>MDFKYTEEKELIKINNVMIHKYTILYTSNCILDISFGEDKITCFNNRLVFLERGVNISVRIQKQKLT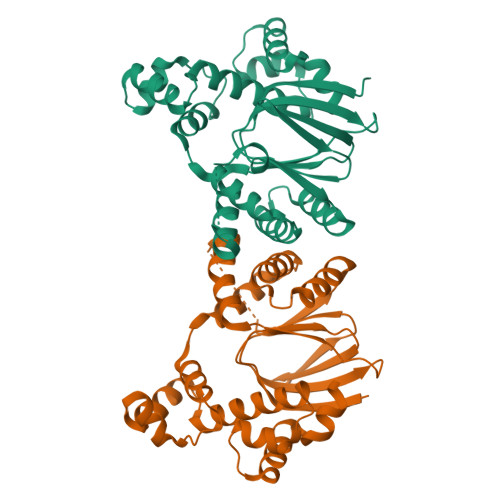EKPYVAFRLNENVLRHLKNTLMIIYGMSKIDSCECRGVSRKIMTTEVDKMLLNVLREMMGHHNDDSSFISALIYLISKIKCNDKIIESLYMSSITFFTDKVRGVIEKDLSRKWTLAIIADVFNVSEITIRKRLESEDTNFNQILMQSRMSKAALLLLENSYQISQISNMIGISSASYFIRIFNKHFGVTPKQFFNYFKGG[2x]> IKELKMSKDEIKREYKEMEGSPEIKSKRRQFHQEIQSGNMRENVKRSSVVVAAPTHIAIGILYKRGETPLPLVTFKYTDAQVQTVRKIAEEEGVPILQRIPLARALYWDALVDHYIPAEQIEATAEVLRWLERQNI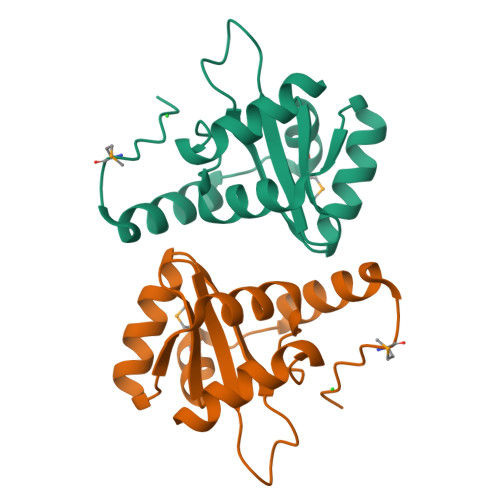EKQHSEML> SNAMRIVVALGGNALLRRGEPMTADNQRENVRIAAEQIAKVAPGNELVIAHGNGPQVGLLALQGAAYDKVSPYPLDVLGAETEGMIGYMIEQEMGNLLPFEVPFATILTQVEVDGKDPAFQNPTKPIGPVYSREEAERLAAEKGWSITPDGDKFRRVVPSPRPKRIFEIRPVKWLLEKGTIVICAGGGGIPTMYDEAGKKLSGVEAVIDKDLCSSLLAQELVADIL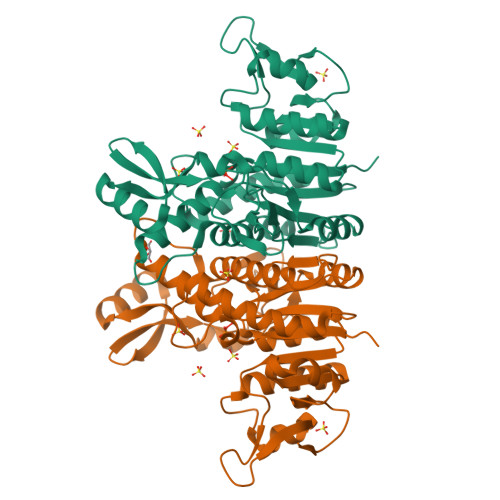IIATDVDAAYVDWGKPTQKAIAQAHPDELERLGFAAGSMGPKVQAAIEFARATGKDAVIGSLADIVAITEGKAGTRVSTRKAGIEYR>[2x]MLNSCSMPLGMESKAISDAQITASSYACRGDTCWSPSKARLHLQGRSNAWRPQVNNPKEWLQVDFQKTMKVTGVTTQGVKSAATSMYVKEFLISSSQDGHQWTLFFQNGKVK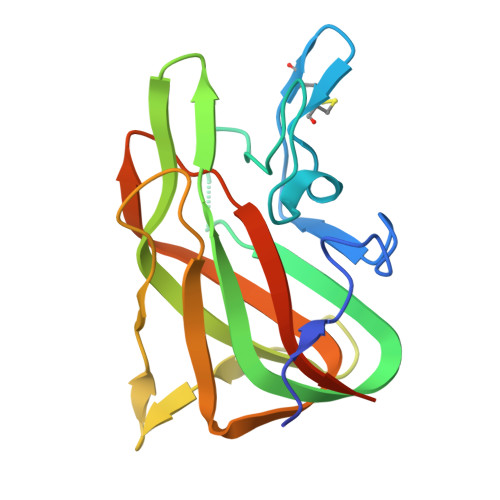VFQGNQDSFTPVVNSLDPPLLTRYLRIHPQSWVHQIALRMEVLGCEAQDLYENLYFQ>[4x]MAEFRIAQDVVARENDRRASALKEDYEALGANLARRGVDIEAVTAKVEKFFVAVPSWGVGTGGTRFARFPGTGEPRGIFDKLDDCAVIQQLTRATPNVSLHIPWDKADPKELKARGDALGLGFDAMNSNT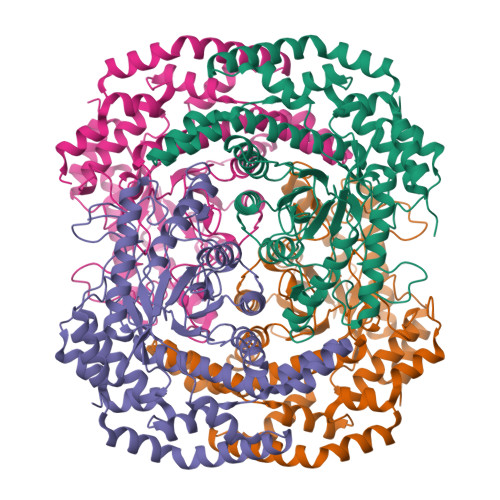FSDAPGQAHSYKYGSLSHTNAATRAQAVEHNLECIEIGKAIGSKALTVWIGDGSNFPGQSNFTRAFERYLSAMAEIYKGLPDDWKLFSEHKMYEPAFYSTVVQDWGTNYLIAQTLGPKAQCLVDLGHHAPNTNIEMIVARLIQFGKLGGFHFNDSKYGDDDLDAGAIEPYRLFLVFNELVDAEARGVKGFHPAHMIDQLHNVTDPIESLINSANEIRRAYAQALLVDRAALSGYQEDNDALMATETLKRAYRTDVEPILAEARRRTGGAVDPVATYRASGYRARVAAERPASVAGGGGIIGSHHHHHH> HGDPKVVE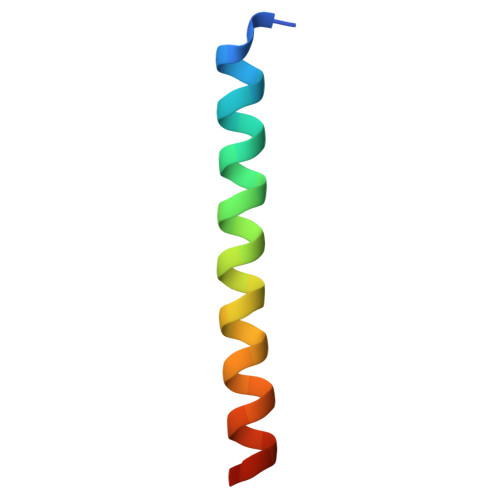TYVELLKRHEKAVKELLEIAKTHAKKVE>ALTAKHRPSVVWLHNAECTGCTEAAIRTIKPYIDALILDTISLDYQETIMAAAGEAAEAALHQALEGKDGYYLVVEGGLPTIDGGQWGMVAGHPMIETTKKAAAKAKGIICIGTCSAYGGVQKAKPNPSQAKGVSEALGVKTINIPGCPPNPINFVGAVVHVLTKGIPDLDENGRPKLFYGELVHDNCPRLPHFEASEFAPSFDSEEAKKGFCLYELGCKGPVTYNNCPKVLFNQVNWPVQAGHPCLGCSEPDFWDTMTPFYEQG[2x];>ASWSHPQFEKGASGAAESKPTPQSTFTGPIVVDPITRIEGHLRIMVEVENGKVKDAWSSSQLFRGLEIILKGRDPRDAQHFTQRACGVCTYVHALASSRCVDDAVKVSIPANARMMRNLVMASQYLHDHLVHFYHAHALDWVDVTAALKADPNKAAKLAASIAPARPGNSAKALKAVQDKLKAFVESGQLGIFTNAYFLGGHKAYYLPPEVDLIATAHYLEALHMQVKAASAMAILGGKNPHTQFTVVGGCSNYQGLTKDPLANYLALSKEVCQFVNECYIPDLLAVAGFYKDWGGIGGTSNYLAFGEF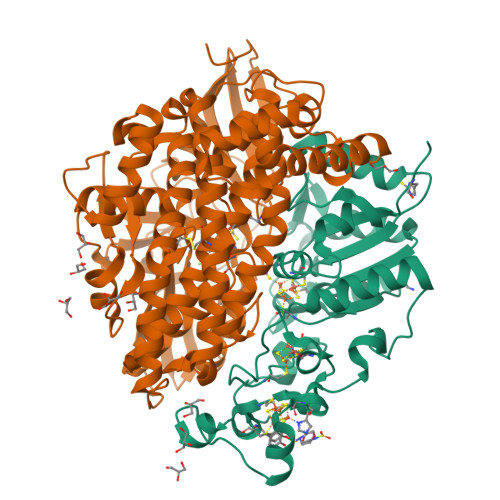ATDDSSPEKHLATSQFPSGVITGRDLGKVDNVDLGAIYEDVKYSWYAPGGDGKHPYDGVTDPKYTKLDDKDHYSWMKAPRYKGKAMEVGPLARTFIAYAKGQPDFKKVVDMVLGKLSVPATALHSTLGRTAARGIETAIVCANMEKWIKEMADSGAKDNTLCAKWEMPEESKGVGLADAPRGALSHWIRIKGKKIDNFQLVVPSTWNLGPRGAQGDKSPVEEALIGTPIADPKRPVEILRTVHAFDPCIACGVH[2x]1-(1H-imidazol-1-yl)-4,4-diphenylbutan-2-one | C19 H18 N2 O | 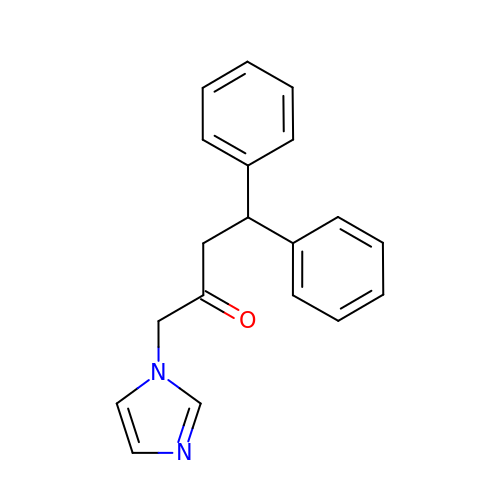SRAWFXXOZVYZRX-UHFFFAOYSA-N> SNAMSSSSSPPHQLNHFSDVANKAANAAGDVIRKYFRKNNFDIIHKNDLSPVTIADQSAEEAMVSVILDNFPSHAVYGEEKGWRCKQDSADYVWVLDPIDGTKSFITGKPLFGTLIALLQNGTPILGIIDQPVLKERWIGITGKRTTLNGQEVSTRTCADLSQAYLYTTSPHLFSGDAEEAFIRVRDKVKIPLYGCDCYAYALLSSGFVDLVVESGLKPYDFLALIPVIEGSGGVITDWKGHQLRWEASPLSIATSFNVVAAGDKQIHQQALDSLQW

The examples shown in the Methods section ascertain that SeU can be successfully and conveniently used as a practical and easily applicable vehicle for phasing novel crystal structures of macromolecules by the SAD (or MAD) approach through the anomalous signal of selenium. The use of SeU as a provider of anomalous signal for the SAD phasing has been examined on crystals of several proteins and a nucleic acid.

The two amide groups of SeU may serve as donors in hydrogen bonds formed with various acceptors, such as carbonyl or carboxyl functions of various amino acids, hydroxyl groups of Thr and Tyr residues or suitable atoms of nucleic acids. On the other hand, the Se atom in the central selenocarbonyl moiety of SeU may accept hydrogen bonds from various donors, provided by amides, hydroxyl groups and protonated amines. The high concentrations of urea are routinely used for denaturation of proteins, but no adverse effects were observed after relatively short exposure of protein crystals to SeU.> SRGRGRRRRLVWTPSQSEALR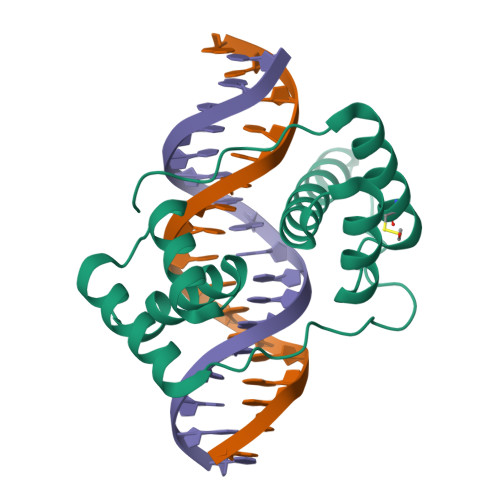ACFERNPYPGIATRERLAQAIGIPEPRVQIWFQNERSRQLRQHRRESRPWPGRRGPPEGRRKRTAVTGSQTALLLRAFEKDRFPGIAAREELARETGLPESRIQIWFQNRRARHPGQGGR2-{(S)-(2-chlorophenyl)[2-(1-methyl-1H-imidazol-2-yl)ethoxy]methyl}-1H-pyrrolo[3,2-b]pyridine-7-carboxylic acid | C21 H19 Cl N4 O3 | 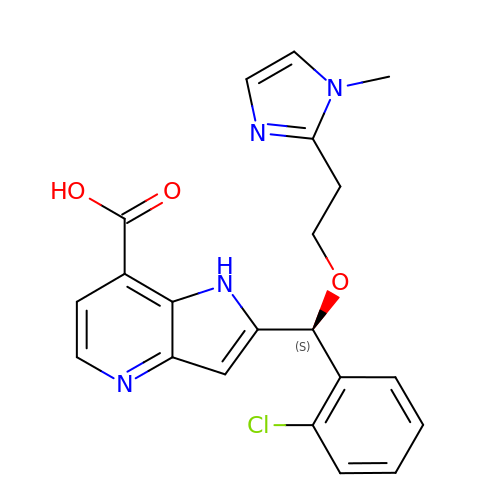ULBCSYUKODTPKF-FQEVSTJZSA-N(3M,4aR,5aR)-3-(1H-tetrazol-5-yl)-4,4a,5,5a-tetrahydro-1H-cyclopropa[4,5]cyclopenta[1,2-c]pyrazole 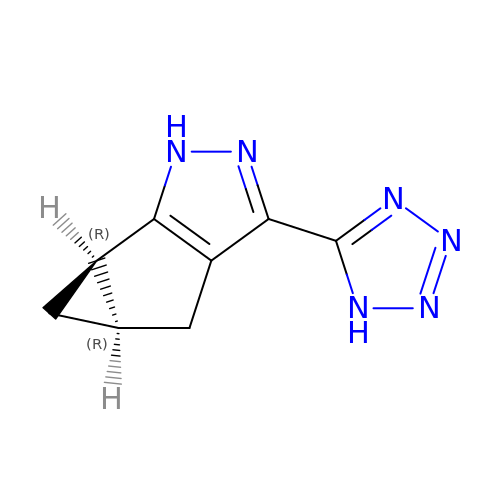| C8 H8 N6 | DKSPRNJUDCWTID-QWWZWVQMSA-N Fragaceatoxin C (FraC)11 is a potent haemolysin of the family of actinoporins, defined as a group of ~20 kDa protein toxins produced by sea anemones. Actinoporins are classified as α-helical PFT (α-PFT) because the transmembrane pore is predicted to form an α-helical barrel. The lytic activity of actinoporins on biological membranes is enhanced by the lipid sphingomyelin (SM) and by lipid-phase coexistence. Here we reveal structures of FraC corresponding to four different stages of its activation route, namely the water-soluble form, the lipid-bound form, an assembly intermediate and the transmembrane pore.

The crystal structure of a dimeric form of FraC in two crystal forms at 1.57 and 1.60 Å resolution sheds light on the initial events leading to the assembly of the pore. These two high-resolution crystal structures are virtually identical to each other. Suitable crystals were obtained in the presence of POC (a compound that mimics the lipid headgroup of DOPC and SM) and the detergent dodecyl-β-maltoside (DDM). Two molecules of POC are bound to each protein chain, occupying identical positions to those of the headgroups of lipids L2 and L3 in the crystal structure of both, the transmembrane pore and the DHPC-bound monomer. The protein–protein dimerization surface and the non-covalent interactions observed in the dimer resemble those between residues of the β-core region in the transmembrane pore (rmsd=0.4±0.04 Å). The structure of the dimer reveals a localized and notable conformational change with respect to the monomer (water soluble) at residues 14–17 of the N-terminal region. In the monomeric form of FraC, the side chain of Phe16 is inserted in a hydrophobic cavity of the β-core region. In contrast, during dimerization the residue Val60 of a second protein chain displaces Phe16 from its original position, leading to (i) partial unfolding and increase strain in the peptide bond of Phe16 and its neighbouring residue Leu14, (ii) a displacement of 4.7±0.1 Å of the Cα of Phe16 towards the solvent and (iii) further structural adjustments of Gly15 and Asp17. Because the N-terminal region is glued to the β-core region, partly by interactions between apolar residues, the rearrangement of two large hydrophobic residues (Leu14 and Phe16) may facilitate the detachment of the N-terminal region towards the membrane, a necessary condition to generate the active pore. Second, the serendipitous capture of a dimeric form of FraC exhibiting a similar protein–protein interaction interface to that of the pore, suggests a mechanism initiating the self-assembly and metamorphosis of FraC.

>SADVAGAVIDGAGLGFDVLKTVLEALGNVKRKIAVGIDNESGKTWTAMNTYFRSGTSDIVLPHKVAHGKALLYNGQKNRGPVATGVVGVIAYSMSDGNTLAVLFSVPYDYNWYSNWWNVRVYKGQKRADQRMYEELYYHRSPFRGDNGWHSRGLGYGLKSRGFMNSSGHAILEIHVTKA[2x]> QQYKTFMGARVLWPPECADDILEGAIRETQDALKKFEIAREGQKIAEHLKKYMDDHFDPYWHVF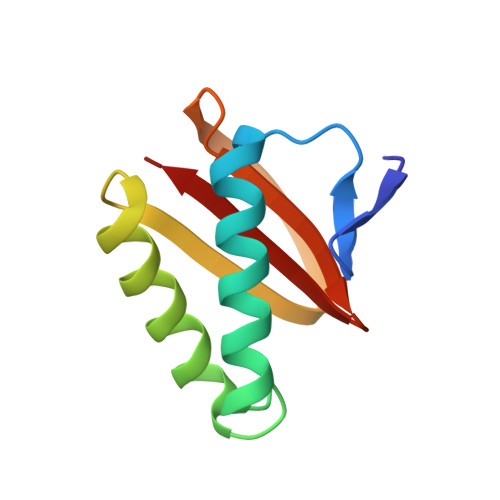FGKNFGCQAVHNKNRFIYFYIEKTAFLMYQT YTHDF proteins bind the N6-methyladenosine (m6A)-modified mRNAs, influencing their processing, stability, and translation. YTHDF proteins contain a hydrophobic pocket that accommodates the m6A embedded in the RRACH consensus sequence on mRNAs. The YTH domains of YTHDF1, DF2, and DF3 share a common fold with a central β-sheet surrounded by five α-helices. Three conserved tryptophan residues largely define the hydrophobic pocket involved in m6A binding.

To further study the ebselen binding and mode, the YTH domain of the YTHDF1 protein was co-crystallized with ebselen, and X-ray diffraction data were collected at the Se absorption edge to locate the Se atom unambiguously. The Se atom appeared to be involved in a covalent bond with Cys412. The ebselen molecule sits on a very shallow groove with one side resting on the locally hydrophobic protein matrix, while the other face remains solvent-exposed. However, in the two protein chains in the asymmetric unit, ebselen preferentially adopts two slightly different poses. In the first case, the selenobenzene moiety almost inserts between the aliphatic segments of the Lys471 and Lys473 side chains while also contacting the intervening Gly472; the N-phenyl amide group stacks to Tyr408 concurrently interacting with the Arg404 and Ile410 side chains. In the other pose, while the selenobenzene group maintains similar interactions with a minor ring rotation (32°), the N-phenylformamide moiety inserts more deeply into the groove in van der Waals contact to Asp401, Arg404, Ser405, Ile410, and Trp411. Electron density is missing for a relevant part of the extended β4−β5 loop (residues 460–469), which is then flexible and disordered. Although binding at a site different from the m6A pocket, the ebselen molecule impedes the conformational rearrangement of the β4−β5 loop into the m6A-binding-competent conformation. The selenobenzene ring in both ebselen poses clashes with YTHDF1 residues Ser461–Ala462 in the m6A-bound structure, while the N-phenylformamide group either collides with Trp465 or Val464. Finally, ebselen displacement of both Trp465 and Trp470 generates a unique pocket extending to the m6A-binding region that can be exploited by ebselen derivatives with improved potency.

>[2x]GSVESHPVLEKLKAAHSYNPKEFEWNLKSGRVFIIKSYSEDDIHRSIKYSIWCSTEHGNKRLDSAFRCMSSKGPVYLLFSVNGSGHFCGVAEMKSPVDYGTSAGVWSQDKWKGKFDVQWIFVKDVPNNQLRHIRLENNDNKPVTNSRDTQEVPLEKAKQVLKIISSYKHTTSIFDDFAHYEKRQAVVEVVRKERQSRNKQ> PVDFNGYWKMLSNENFEEYLRALDVNVALRKIANLLKPDKEIVQDGDHMIIRTLSTFRNYIMDFQVGKEFEEDLT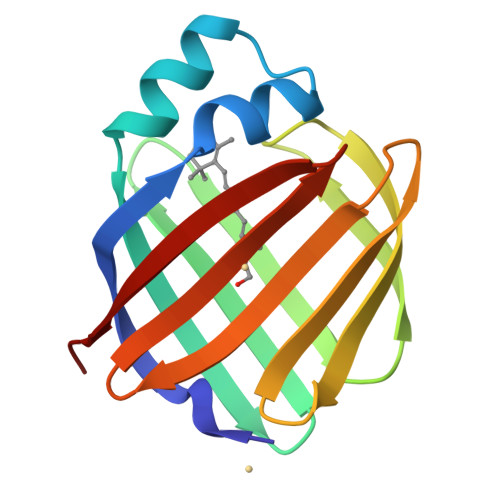GIDDRKCMTTVSWDGDKLQCVQKGEKEGRGWTQWIEGDELHLEMRAEGVTCKQVFKKVH The hyperthermophilic endocellulase, EGPh (glycosyl hydrolase family 5) from Pyrococcus horikoshii possesses 4 cysteine residues forming 2 disulfide bonds, as identified by structural analysis. The crystal structure of hyperthermophilic beta-1,4 endocellulases (EGPh, glycosyl hydrolase family 5, T opt = 100 °C) from the archaeon Pyrococcus horikoshii, that was isolated from an oceanic hydrothermal volcanic vent, has been determined. The crystal structure of EGPh revealed 4 Cys residues (C106, C159, C372, and C412) forming 2 disulfide bonds. The disulfide bonding of C106 and C159 forms at the end of the loop associated with the substrate-binding active site cleft.

To investigate a role of the disulfide bond in the activity and stability of the enzyme, we prepared 3 mutants of EGPh; P74C, C106S, and P74C/C106S, in which we removed the disulfide bond or changed the disulfide-bonding pattern. In the mutant P74C, we paid particular attention to which pair of residues among the 3 Cys residues (C74, C106, and C159) would participate in disulfide bond formation in EGPh. The structural data demonstrated that the substituted C74 residue formed a new disulfide bond (C74–C159). The newly formed disulfide bond (C74–C159) in EGPh was located at the conserved position for the disulfide bond (C34–C120) in EGAc. The conformation of the newly formed disulfide bond in EGPh also exactly matched with that of EGAc on the superimposed structure. The neighboring residues around the Cys residues were not affected structurally by the mutation. The structure of P74C with 3 Cys residues near the active site showed the same disulfide-bonding pattern as that of EGAc, suggesting that the conserved C159 prefers a linkage with the substituted C74 rather than with C106, unlike that of the wild type. The Cα–Cα distance (5.0 Å) of C74–C159 was also slightly closer (5.7 Å) than that of C106–C159. These structural factors may allow the conserved residue C159 to easily form a disulfide bond with the substituted C74 rather than C106 of the wild type. The wild type enzyme was thermally unfolded at 103.4 °C. The melting temperature of the 3 mutants was approximately 101.5 °C. These results indicate that the alternative new disulfide-bonding pattern involved in the position of P74 did not contribute to its hyperthermostability.

>[3x]QTPTGIYYEVRGDTIYMINVTSGEETPIHLFGVNWFGFETPNHVVHGLWKRNWEDMLLQIKSLGFNAIRLPFCTESVKPGTQPIGIDYSKNPDLRGLDSLQIMEKIIKKAGDLGIFVLLDYHRIGCTHIEPLWYTEDFSEEDFINTWIEVAKRFGKYWNVIGADLKNEPHSVTSPPAAYTDGTGATWGMGNPATDWNLAAERIGKAILKVAPHWLIFVEGTQFTNPKTDSSYKWGYNAWWGGNLMAVKDYPVNLPKNKLVYSPHVYGPDVYNQPYFGPAKGFPDNLPDIWYHHFGYVKLELGYSVVIGEFGGKYGHGGDPRDVIWQNKLVDWMIENKFCDFFYWSWNPDSGDTGGILQDDWTTIWEDKYNNLKRLMD> NVG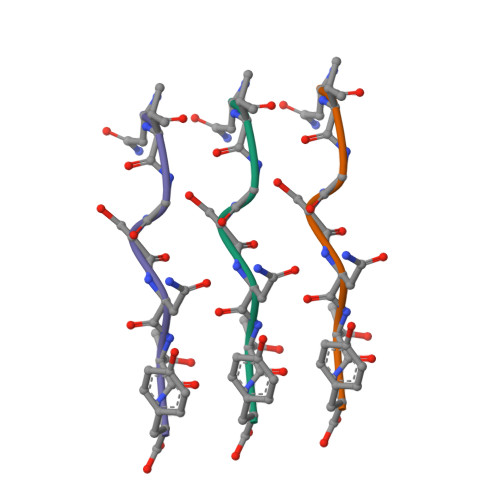SNTY> MLVWLAEHLVKYYSGFNVFSYLTFRAIVSLLTALFISLWMGPRMIAHLQKLSFGQVVRNDGP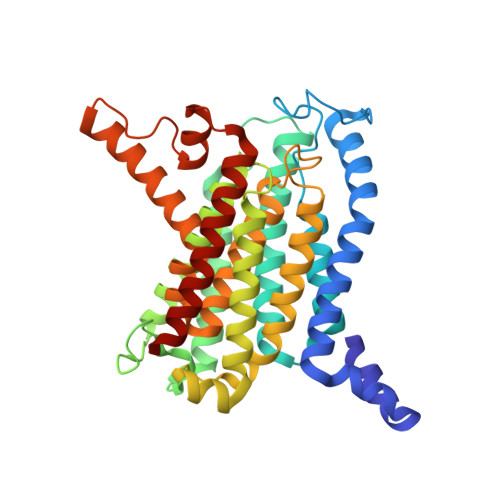ESHFSKRGTPTMGGIMILTAIVISVLLWAYPSNPYVWCVLVVLVGYGVIGFVDDYRKVVRKDTKGLIARWKYFWMSVIALGVAFALYLAGKDTPATQLVVPFFKDVMPQLGLFYILLAYFVIVGTGNAVNLTDGLDGLAIMPTVFVAGGFALVAWATGNMNFASYLHIPYLRHAGELVIVCTAIVGAGLGFLWFNTYPAQVFMGDVGSLALGGALGIIAVLLRQEFLLVIMGGVFVVETLSVILQVGSFKLRGQRIFRMAPIHHHYELKGWPEPRVIVRFWIISLMLVLIGLATLKVR>MNIHEWQSKQLIQKYGGRAQSGEVAFSPERSRDIAKKLWNQFPGCEFVVKAQVLAGGRGKGHWEHGMQGGVKLAKTPEEVYEIANEMIGHKLITKQTGAKGINCNKVMVCGAVDILKEFYLSILLDRAMGCP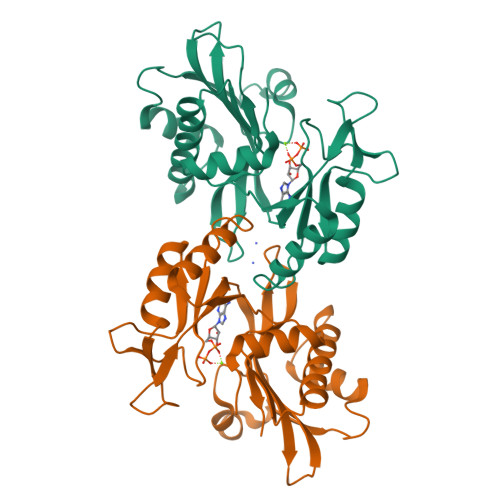VIIATSQGGMGIEEVAQKCPECLFKVPISVKNGPTNEQLVKLAKDLGLEGDLVQDCVDNVKALYQVFDKCDSTMVEINPLGVIETPTDEKVICCLDAKIAFDKDAAFGLEHHHHHHHH[4x]>[2x]LLEQEDVVEMDDNFEFGLCPCDAKPIVRGKFNTTLLNGPAFQMVCPIGWTGTVSCTSFNMDTLATTVVRTYRRSKPFPHRQGCITQKNLGEDLHNCILGGNWTCVPGDQLLYKGGSIESCKWCGYQFKESEGLPHYPIGKCKLENETGYRLVDSTSCNREGVAIVPQGTLKCKIGKTTVQVIAMDTKLGPMPCRPYEIISSEGPVEKTA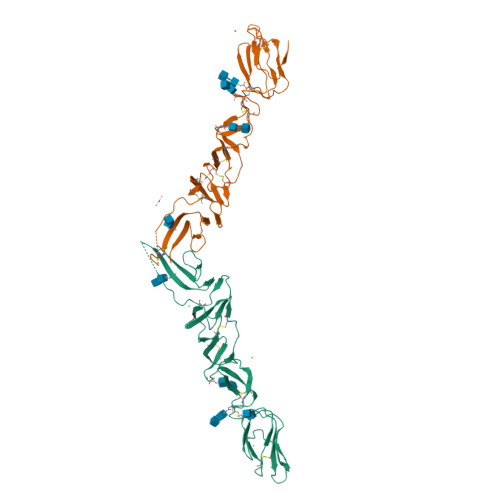CTFNYTKTLKNKYFEPRDSYFQQYMLKGEYQYWFDLEVTDHHRD>LPEQIDWRKKGAVTPVKNQGSCGSCWAFSTVSTVESINQIRTGNLISLSEQELVDCDKKNHGCLGGAFVFAYQYIINNGGIDTQANYPYKAVQGPCQAASKVVSIDGYNGVPFCNEXALKQAVAVQPSTVAID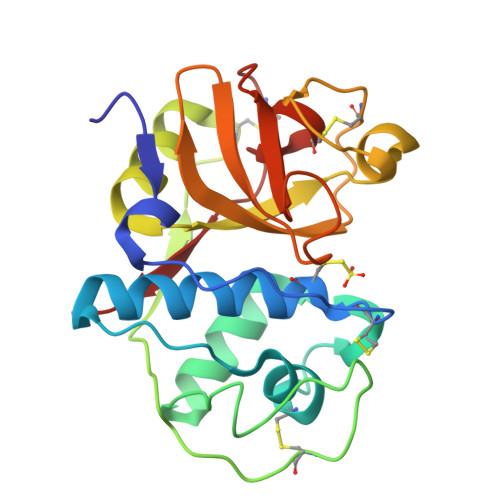ASSAQFQQYSSGIFSGPCGTKLNHGVTIVGYQANYWIVRNSWGRYWGEKGYIRMLRVGGCGLCGIARLPYYPTKA[2x]5-methyl-3~{H}-furan-2-one | C5 H6 O2 | 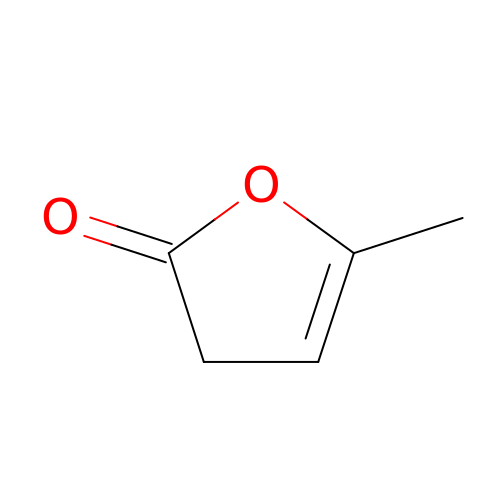QOTQFLOTGBBMEX-UHFFFAOYSA-N>[2x]MSKRPNFLVIVADDLGFSDIGTFGGEIATPNLDALAIAGLRLTDFHTASAASPTRSMLLTGTDHHIAGIGTMAEALTPELEGKPGYE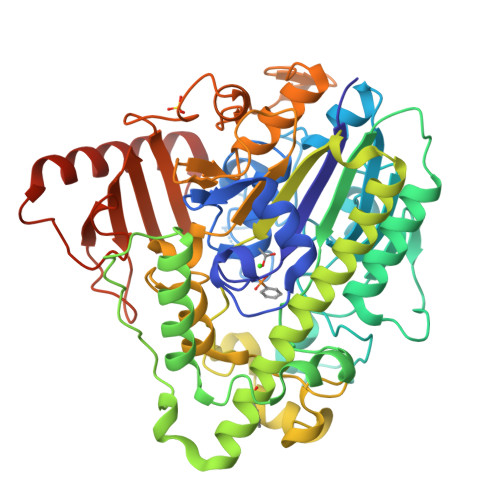GHLNERVVALPELLREAGYQTLMAGKWHLGLKPEQTPHARGFERSFALLPGAANHYGFEPPYDESTPRILKGTPALYVEDERYLDTLPEGFYSSDAFGDKLLQYLKERDQSRPFFAYLPFSAPHWPLQAPREIVEKYRGRYDAGPEALRQERLARLKELGLVEADVEAHPVLALTREWEALEDEERAKSARAMEVYAAMVERMDWNIGRVVDYLRRQGELDNTFVLFMSDNGAEGALLEAFPKFGPDLLDFLDRHYDNSLENIGRANSYVWYGPRWAQAATAPSRLYKAFTTQGGIRVPALVRYPRLSRQGAISHAFATVMDVTPTLLDLAGVRHPGKRWRGREIAEPRGRSWLGWLSGETEAAHDENTVTGWGLFGMRAIRQGDWKAVYLPAPVGPATWQLYDLARDPGEIHDLADSQPGKLAELIEHWKRYVSDTGVVEGASPFLVR> SNAKILAVTACPTGIAHTFMAADALKEKAKELGVEIKVETNGSSGIKHKLTAQEIEDAPAIIVAADKQVEMER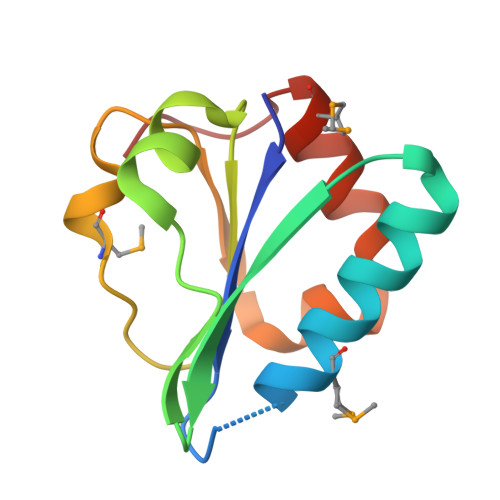FKGKRVLQVPVTAGIRRPQELIEKAMNQDAPIY> SMTDLLSAEDIKKAIGAFTAAD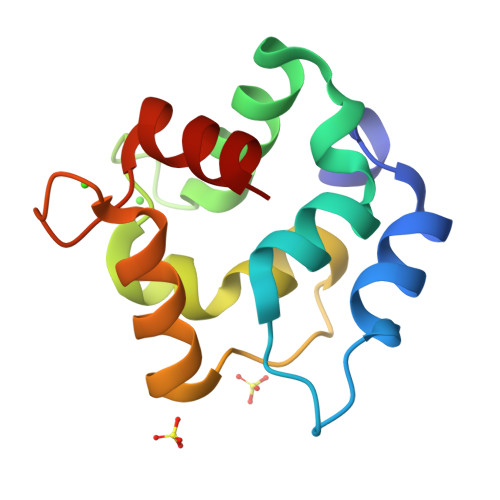SFDHKKFFQMVGLKKKSADDVKKVFHILDKDKSGFIEEDELGSILKGFSSDAADLSAKETKTLMAAGDKDGDGKIGVEEFSTLVAES> MI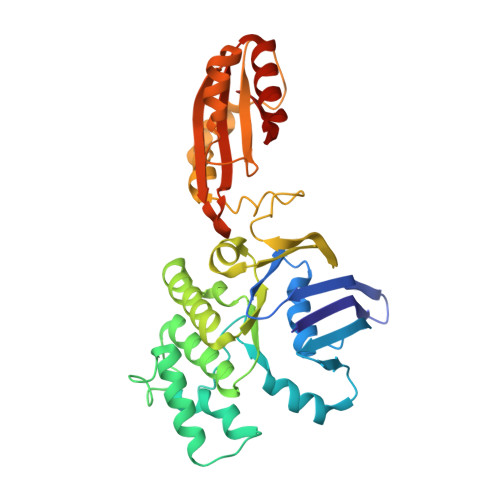KLSNITKVFHQGTRTIQALNNVSLHVPAGQIYGVIGASGAGKSTLIRCVNLLERPTEGSVLVDGQELTTLSESELTKARRQIGMIFQHFNLLSSRTVFGNVALPLELDNTPKDEVKRRVTELLSLVGLGDKHDSYPSNLSGGQKQRVAIARALASNPKVLLCDEATSALDPATTRSILELLKDINRRLGLTILLITHEMDVVKRICDCVAVISNGELIEQDTVSEVFSHPKTPLAQKFIQSTLHLDIPEDYQERLQAEPFTDCVPMLRLEFTGQSVDAPLLSETARRFNVNNNIISAQMDYAGGVKFGIMLTEMHGTQQDTQAAIAWLQEHHVKVEVLGYV>GPMKTEMKDDFAKLEEQFDAKLGIFALDTGTNRTVAYRPDERFAFASTIKALTVGVLLQQKSIEDLNQRITYTRDDLVNYNPIT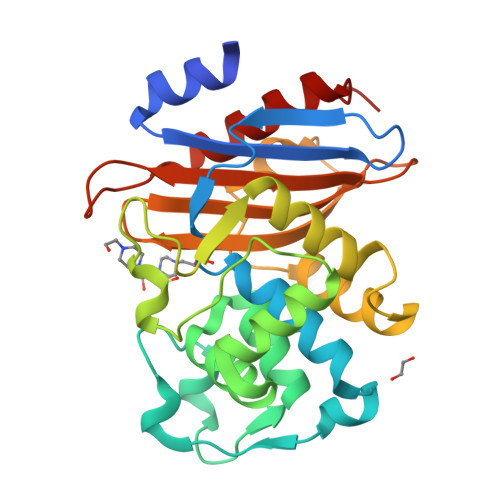EKHVDTGMTLKELADASLRYSDNAAQNLILKQIGGPESLKKELRKIGDEVTNPERFYPELNEVNPGETQDTSTARALVTSLRAFALEDKLPSEKRELLIDWMKRNTTGDALIRAGVPDGWEVADKTGAASYGTRNDIAIIWPPKGDPVVLAVLSSRDKKDAKYDDKLIAEATKVVMKALNMNGK[2x]>[2x]CTACGGCCG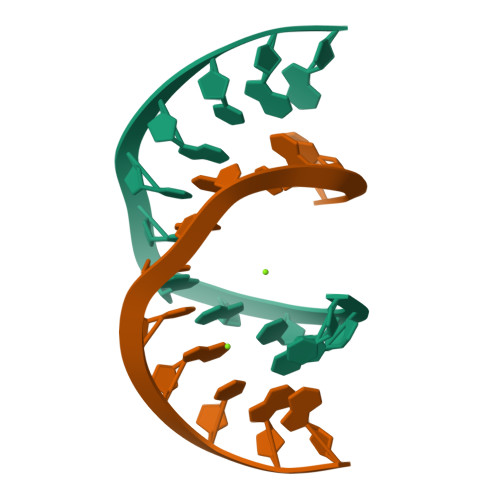TAG(4S)-N-[3-(1,3-oxazol-5-yl)phenyl]-7-[3-(trifluoromethyl)phenyl]-3,4-dihydro-1,4-methanopyrido[2,3-b][1,4]diazepine-5(2H)-carboxamide 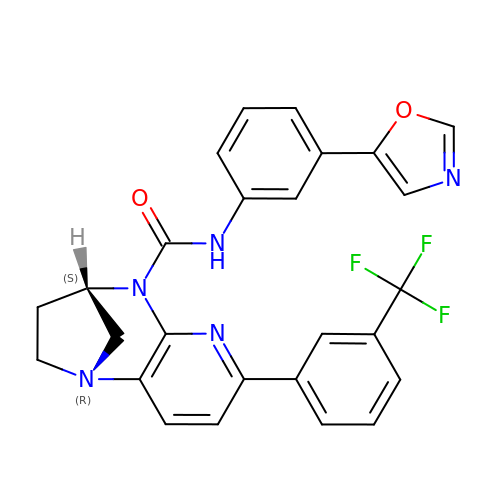| C26 H20 F3 N5 O2 | DNDUUAHYXRIMOM-FQEVSTJZSA-N>RKCLNTPLPLIYTTCPIGQDKCV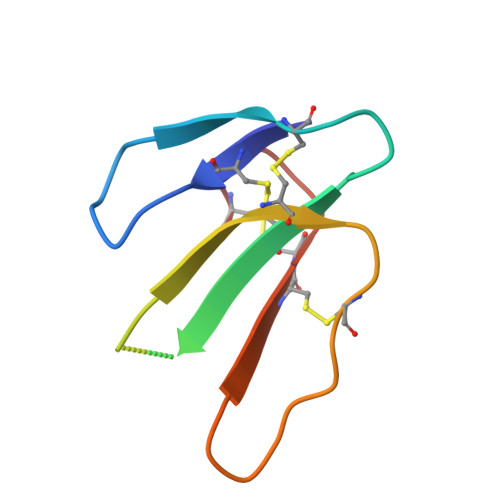KMTIKKLPSKYDVIRGCIDICPKSSADVEVLCCDTNKCNK[3x]> MEDVEIKPRGYQLRLVDHLTKSNGIVYLPTGSGKTFVAILVLKRFSQDFDKPIESGGKRALFMCN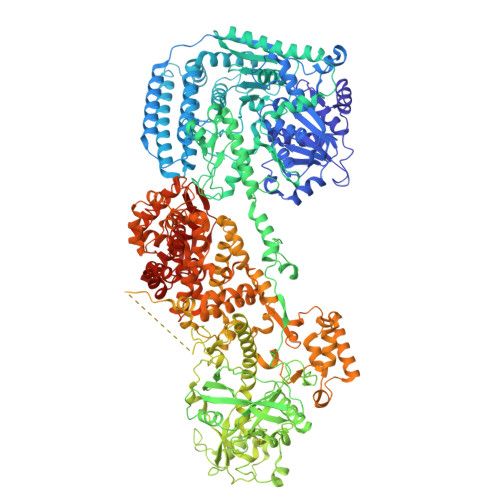TVELARQQAMAVRRCTNFKVGFYVGEQGVDDWTRGMWSDEIKKNQVLVGTAQVFLDMVTQTYVALSSLSVVIIDECHHGTGHHPFREFMRLFTIANQTKLPRVVGLTGVLIKGNEITNVATKLKELEITYRGNIITVSDTKEMENVMLYATKPTEVMVSFPHQEQVLTVTRLISAEIEKFYVSLDLMNIGVQPIRRSKSLQCLRDPSKKSFVKQLFNDFLYQMKEYGIYAASIAIISLIVEFDIKRRQAETLSVKLMHRTALTLCEKIRHLLVQKLQDMTYDDDDDNVNTEEVIMNFSTPKVQRFLMSLKVSFADKDPKDICCLVFVERRYTCKCIYGLLLNYIQSTPELRNVLTPQFMVGRNNISPDFESVLERKWQKSAIQQFRDGNANLMICSSVLEEGIDVQACNHVFILDPVKTFNMYVQSKGRARTTEAKFVLFTADKEREKTIQQIYQYRKAHNDIAEYLKDRVLEKTEPELYEIKGHFQDDIDPFTNENGAVLLPNNALAILHRYCQTIPTDAFGFVIPWFHVLQEDERDRIFGVSAKGKHVISINMPVNCMLRDTIYSDPMDNVKTAKISAAFKACKVLYSLGELNERFVPKTLKERVASIADVHFEHWNKYGDSVTATVNKADKSKDRTYKTECPLEFYDALPRVGEICYAYEIFLEPQFESCEYTEHMYLNLQTPRNYAILLRNKLPRLAEMPLFSNQGKLHVRVANAPLEVIIQNSEQLELLHQFHGMVFRDILKIWHPFFVLDRRSKENSYLVVPLILGAGEQKCFDWELMTNFRRLPQSHGSNVQQREQQPAPRPEDFEGKIVTQWYANYDKPMLVTKVHRELTPLSYMEKNQQDKTYYEFTMSKYGNRIGDVVHKDKFMIEVRDLTEQLTFYVHNRGKFNAKSKAKMKVILIPELCFNFNFPGDLWLKLIFLPSILNRMYFLLHAEALRKRFNTYLNLHLLPFNGTDYMPRPLEIDYSLKRNVDPLGNVIPTEDIEEPKSLLEPMPTKSIEASVANLEITEFENPWQKYMEPVDLSRNLLSTYPVELDYYYHFSVGNVCEMNEMDFEDKEYWAKNQFHMPTGNIYGNRTPAKTNANVPALMPSKPTVRGKVKPLLILQKTVSKEHITPAEQGEFLAAITASSAADVFDMERLEILGNSFLKLSATLYLASKYSDWNEGTLTEVKSKLVSNRNLLFCLIDADIPKTLNTIQFTPRYTWLPPGISLPHNVLALWRENPEFAKIIGPHNLRDLALGDEESLVKGNCSDINYNRFVEGCRANGQSFYAGADFSSEVNFCVGLVTIPNKVIADTLEALLGVIVKNYGLQHAFKMLEYFKICRADIDKPLTQLLNLELGGKKMRANVNTTEIDGFLINHYYLEKNLGYTFKDRRYLLQALTHPSYPTNRITGSYQELEFIGNAILDFLISAYIFENNTKMNPGALTDLRSALVNNTTLACICVRHRLHFFILAENAKLSEIISKFVNFQESQGHRVTNYVRILLEEADVQPTPLDLDDELDMTELPHANKCISQEAEKGVPPKGEFNMSTNVDVPKALGDVLEALIAAVYLDCRDLQRTWEVIFNLFEPELQEFTRKVPINHIRQLVEHKHAKPVFSSPIVEGETVMVSCQFTCMEKTIKVYGFGSNKDQAKLSAAKHALQQLSKCDA> GSGELNVSPFVFRENVMVGEKVTATCTTVTEDAQISFKWFKNGKQINDNEHIKVLYYTDFSLLSINPVKADDSGNYTCVITAKEKSSKFTATLTVKASPEWLIQPENVESVMGSNISLQCSVTGIPTPTINWKKSETSSGTDFKSLSTSSNAIILPGGTLNLLRIIKSDEGLYECQASNGIGNDLRKTVTISVFIP

Recently, a shortened Dscam (sDscam) gene family with tandemly arrayed 5′ cassettes in Chelicerata species has been identified, which encodes ∼50–100 isoforms. Chelicerata sDscams could be classified into two subfamilies, sDscamα and sDscamβ, containing one and two variable Ig domains, respectively. Crystal structures and cell aggregation assays demonstrated that both α and β subfamilies of sDscam used Ig1 for the isoform-specific trans recognition in a hand-in-hand manner. Furthermore, the cis interactions were established by the three FNIII domains of sDscam, which assemble into a cross fold with a kink between FNIII2 and FNIII3.

The trans interactions of Chelicerata sDscam were mediated exclusively through the Ig1 domain for both sDscamα and sDscamβ subfamilies. It is worth noting that sDscamβ subfamily has two variable Ig domains, Ig1 and Ig2. The crystal structures of sDscam Ig1 from both M. martensii and L. polyphemus revealed a common assembly of antiparallel homodimer for both α and β subfamilies of sDscam. Similarly, sDscam Ig1 also employs the ABED face to form an antiparallel homodimer. However, among the seven Ig1 structures reported here, the complementary electrostatic potential surface pattern (negative in one end, neutral in the middle, and positive in the other end) has been only observed in the three β isoforms, but not in any one of the four α isoforms.>[4x]PETEEISKGLEDVNIKWTRLTTIDGNKGILRYGGYSVEDIIASGAQDEEIQYLFLYGNLPTEQELRKYKETVQKGYKIPDFVINAIRQLPRESDAVAMQMAAVAAMAASET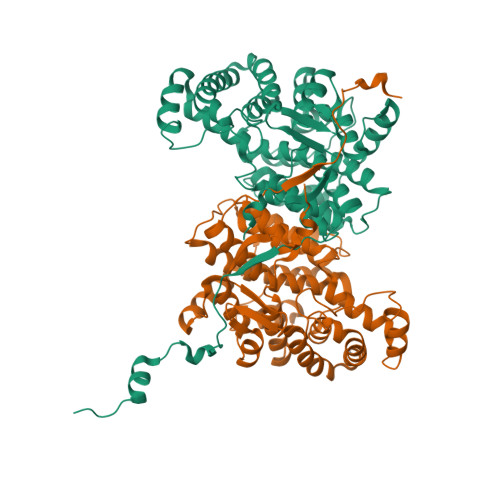KFKWNKDTDRDVAAEMIGRMSAITVNVYRHIMNMPAELPKPSDSYAESFLNAAFGRKATKEEIDAMNTALILYTDHEVPASTTAGLVAVSTLSDMYSGITAALAALKGPLHGGAAEAAIAQFDEIKDPAMVEKWFNDNIINGKKRLMGFGHRVYKTYDPRAKIFKGIAEKLSSKKPEVHKVYEIATKLEDFGIKAFGSKGIYPNTDYFSGIVYMSIGFPLRNNIYTALFALSRVTGWQAHFIEYVEEQQRLIRPRAVYVGPAERKYVPIAERKVDKLAAALEHHHHHH>MKKSLIALTTALSFGLAAAQTAAPVSAPQVPALTDVPAGHWAKDAIDRLVSRGVILGYPDGTFRGTQNLTRYEAAIIIARLLDQMRDGETPAGMTAEDMTALQNAIQELAADLAALGVRVSDLEANAVSKDDFARLEARIEEVAAAGGEQGATEALQGQIDDLTARVDEYDALRADVDDNASSIAALNDLTVLLNQDILDLQDRVSAVEAAQADFVQRSDFDALGGRVTTVETRVETVNNSLTGRIAALERNAFSVKPSLTIGYSVSRTSRNFDVDRLFPLNADGTVANNAFTSGGIDTDTGAQRRDFGDFGNASDPVVAGAAGLYGFADGVSYTVYFTDGSTATFDGLNPADYKVPTGKVIDTTKGRNGFGFNNLARYKEGSTDIGISLGFDTSGQFSQVTSGTGGSLFSTAGRLQVNQIDLNFGLVTGLPSDAYVDTNGNGKKDDGEATGRGTYLGSGGTAAILRDPAGNVYRPVFFRFKNATTQFSVGNNPVIVTLGQQQKFYFSDYVFDNNYDGRGDGFTVTVDGSNVPVIGAWKPQIKGVYGSRSGLDGTAEAGYGVYYRGVRAQITPVGTLTAGIHYAQEGRDMFGAAQNT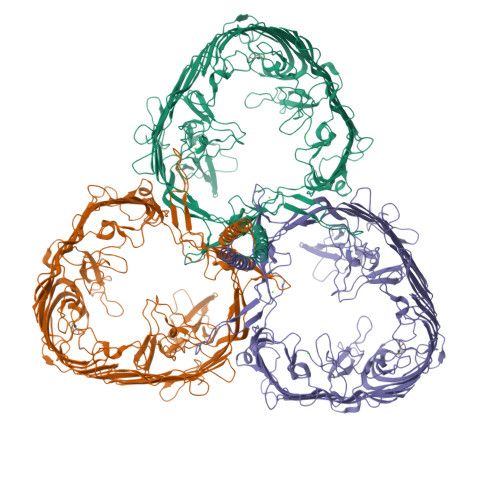TSTPSDVTTYGADLHGKAFGVELHSEYATSRVRPNTANAAVQTSNAFYARVATRKDNLAFDLNTPAAKFGNDTFGVSLYDLNYRKIDAGYNNVAGISEYGYGSYSRTSAQNIAYNPDTGVTAPFANLDRQAYTDANNDGTSDRNADGTVVATNTKIGQMGFGVKAAANLGPVAIGGYYDTSTGANGDNANRMTEAGGSAKVAYSIFSLRGTYNTLDSNRPQIYRDAAGTQIIGDAKVRRYAVQADVTPGLGLFVGAYYRDVNVNGVRSTTDRGLLGRGYLASSFEPGVGNNAYRTGLRCADNNFGTGTRDIDGVGGVLNPAVNLDQSRTATCFTSYGVEAGHAGDNANALVKDLFFRVGYSRVYVPTTATATTGDFSGSVTYGDARYDRKVGVANVRLAGSFSTTNTQLDSRPAGTRGAVGLIVRTDPLENVPFRPQFNGQVGYYTADNRVAAGNYNANATKYGAGVVLNDFLLPQTKIGVRYDGYMAQNRQYTPFDGDGTQGYFSDANNNRRTNLNGVYVEGAYQDLIFSYGTYTLSQKDLNGVEYGSGINNGQPARGQTFKISYKVNF[3x]>SMDPERRVRSTLKKVFGFDSFKTPLQESATMAVVKGNKDVFVCMPTGAGKSLCYQLPALLAKGITIVVSPLIALIQDQVDHLLTLKVRVSSLNSKLSAQERKELLADLEREKPQTKILYITPEMAASSSFQPTLNSLVSRHLLSYLVVDEAHCVSQWGHDFRPDYLRLGALRSRLGHAPCVALTATATPQVQEDVFAALHLKKPVAIFKTPCFRANLFYDVQFKELISDPYGNLKDFCLKALGQEADKGLSGCGIVYCRTREACEQLAIELSCRGVNAKAYHAGL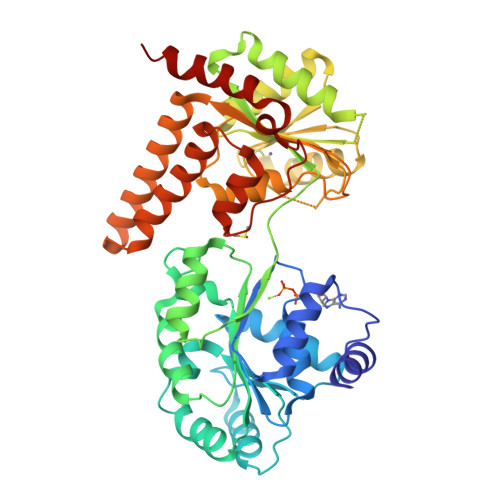KASERTLVQNDWMEEKVPVIVATISFGMGVDKANVRFVAHWNIAKSMAGYYQESGRAGRDGKPSWCRLYYSRNDRDQVSFLIRKEVAKLQEKRGNKASDKATIMAFDALVTFCEELGCRHAAIAKYFGDALPACAKGCDHCQNPTAVRRRLEALERSSSW[4x]> SELYRQSLEIISRYLREQATGAKDTKPMGRSGATSRKALETLRRV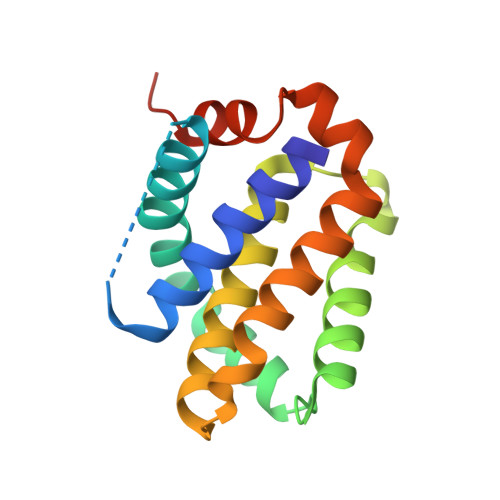GDGVQRNHETAFQGMLRKLDIKNEDDVKSLSRVMIHVFSDGVTNWGRIVTLISFGAFVAKHLKTINQESCIEPLAESITDVLVRTKRDWLVKQRGWDGFVEFFHVEDLEGG> MHHHHHHSSIEGRSMQTQVLFEHPLNEKMRTWLRIEFLIQQLTVNLPIVDHAGALHFFRNVSELLDVFERGEVRTELLKELDRQQRKLQTWIGVPGVDQSRI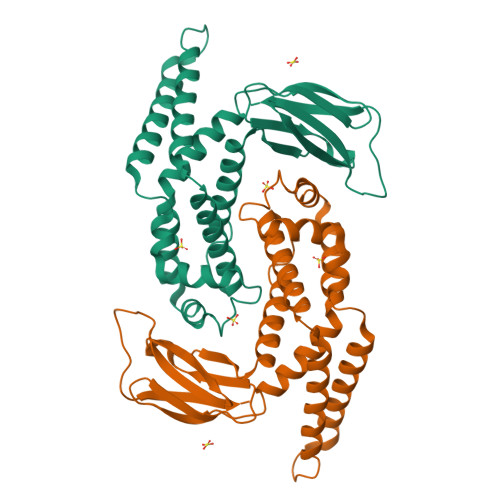EALIQQLKAAGSVLISAPRIGQFLREDRLIALVRQRLSIPGGCCSFDLPTLHIWLHLPQAQRDSQVETWIASLNPLTQALTMVLDLIRQSAPFRKQTSLNGFYQDNGGDADLLRLNLSLDSQLYPQISGHKSRFAIRFMPLDTENGQVPERLDFELACC Methyl 2-(acetylamino)-2-deoxy-1-thio-alpha-D-galactopyranose | C10 H19 N O4 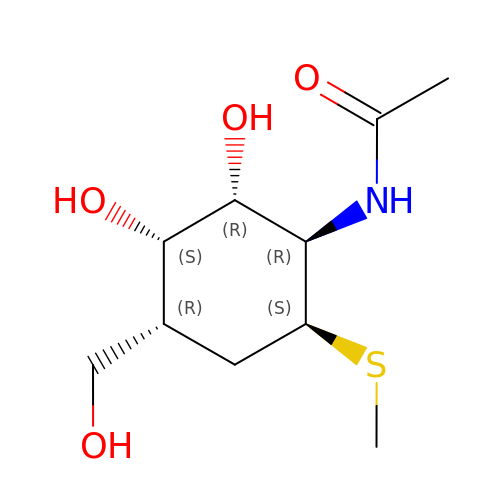S | ZYKRTEHWXBHGOU-SQQIUAQRSA-N> MNKHSGIDFKQLNFLTKLNENHSGEWWKGRWQGNDIVVKVLKVRDWSTRKSRDFNEECPRLRIFSHPNVLPVLGACQSPPAPHPTLITHWMPYGSLYNVLHEGTNFVVDQSQAVKFALDMARGMAFLHTLEPLIPRHALNSRSVMIDEDMTARISMADVKFSFQSPGRMYAPAWVAPEALQKKPEDTNRRSADMWSFAVLLWELVTREVPFADLSNMEIGMKVALEGLRPTIPPGISPHVSKLMKICMNEDPAKRPKFDMIVPILEKMQDK;> GSHMDAFDTLFDHAPDKLNVVKKTLITFVNKHLNKLNLEVTELETQFADGVYLVLLMGLLEGYFVPLHSFFLTPDSFEQKVLNVSFAFELMQDGGLEKPKPRPEDIVNCDLKSTLRVLYNLFTKYR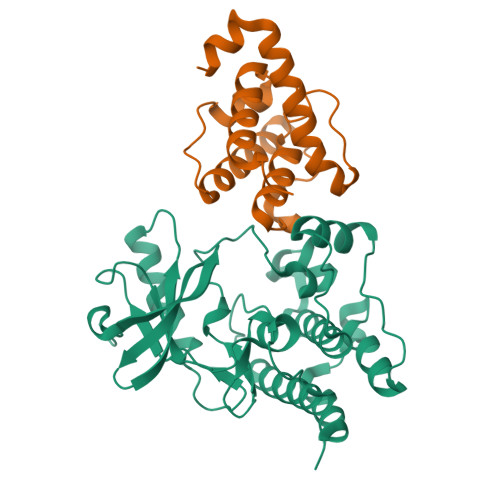NVE N-benzyl-2-[(N-benzyl-beta-alanyl)amino]-4-phenylthiophene-3-carboxamide 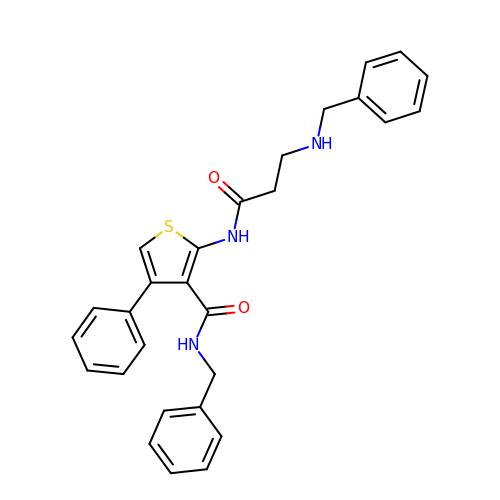| C28 H27 N3 O2 S | WYXRECOQBJBCCU-UHFFFAOYSA-N Isomerization of uridine to its C-glycoside isomer, pseudouridine (Ψ), is the most prevalent RNA modification. Here we address the question of how two homologous E. coli Ψ synthases, RluB and RluF, selectively modify adjacent bases on a stem-loop of E. coli 23S rRNA. RluB is specific for U2605 whereas RluF is selective for U2604, but also modifies U2605 to a small extent. RluB (1–251) is comprised of an N-terminal S4 domain (residues 1–60) connected by a flexible linker to a catalytic domain (residues 66–251).

Escherichia coli RluB (1–251) was co-crystallized with a 21-mer RNA stem-loop identical in sequence to the target stem-loop in 23S rRNA except that U2605 was modified to 5-FU to block the last step in catalysis. Crystals of this complex in space group C2 contained two independent RluB–RNA complexes per asymmetric unit, which are essentially the same with an rmsd of 0.9 Å. The 21-mer RNA stem-loop binds with the target base 5-FU2605 flipped out into the active site cleft and the loop region abutting the S4 domain. The stem-loop has the same secondary structure as it has in the context of the large ribosomal subunit, with A2602 forming a bulge. The target nucleotide, U2605, is flipped into the active site of the enzyme and RluB has turned over 5-FU2605 to give rise to the C1′-C5 glycoside bond typical for Ψ; RluB (1–251) is catalytically active against the 21-mer. But in the RluB structure, one of the RluB–RNA active sites shows clearly that Tyr140, perhaps fortuitously, forms a covalent bond with C6 of the isomerized base. The second RluB–RNA complex is statistically disordered at this site indicating a mixture of covalent and non-covalent complexes. Arg108 intercalates into the stem where U2605 is flipped into the active site, and stacks between base pairs G2588-C2606 and A2590-U2604. RluB stabilizes the bulge with a repertoire of hydrogen bonds involving side chains of His131, Ser133, Glu135 and Arg138, and flips out U2605 into the active site. More likely, stabilizing interactions between the bulge and residues 131–138 connecting α1 and β4 (RluB nomenclature) prevent stem-loop rearrangement in RluB, while absence of such interactions allow rearrangement in RluF.

>[2x]GPGSMSEKLQKVLARAGHGSRREIESIIEAGRVSVDGKIAKLGDRVEVTPGLKIRIDGHLISVRESAEQICRVLAYYKPEGELCTRNDPEGRPTVFDRLPKLRGARWIAVGRLDVNTCGLLLFTTDGELANRLMHPSREVEREYAVRVFGQVDDAKLRDLSRGVQLEDGPAAFKTIKFSGGEGINQWYNVTLTEGRNREVRRLWEAVGVQVSRLIRVRYGDIPLPKGLPRGGWTELDLAQTNYLRELVELPPETS> MTNTLVENIYASVTHNISKKEASK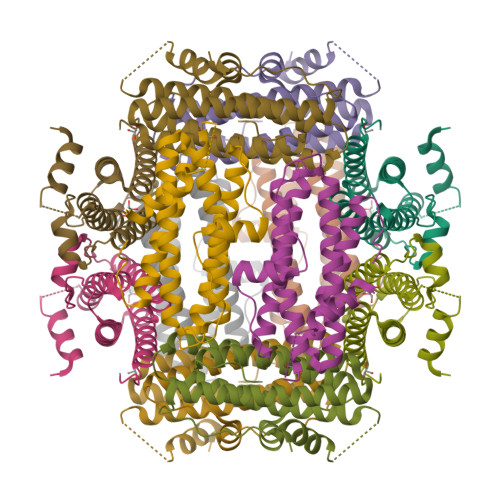NEKTKAVLNQAVADLSVAASIVHQVHWYMRGPGFLYLHPKMDELLDSLNANLDEVSERLITIGGAPYSTLAEFSKHSKLDEAKGTYDKTVAQHLARLVEVYLYLSSLYQVGLDITDEEGDAGTNDLFTAAKTEAEKTIWMLQAERGQGPAL> MSTGITYDEDRKTQLIAQYESVREVVNAEAKNVHVNENASKILLLVVSKLKPASDIQIL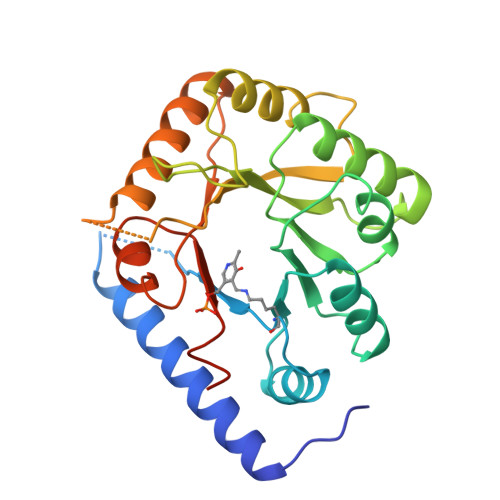YDHGVREFGENYVQELIEKAKLLPDDIKWHFIGGLQTNKCKDLAKVPNLYSVETIDSLKKAKKLNESRAKFQPDCNPILCNVQINTSHEDQKSGLNNEAEIFEVIDFFLSEECKYIKLNGLMTIGSWNVSHEDSKENRDFATLVEWKKKIDAKFGTSLKLSMGMSADFREAIRQGTAEVRIGTDIFGARPPKNEARII> SPTPLPQLPSNVRDGENNVASTFLQAFFQLWDHDRLTLIPQFYDSETTFSVVFATDSPQDPASSSCSKFSRNLNILSPRHPSTLQRLFVGSNLIADLWKVLPATRHPSLDQTSQWLIDCHTFPHLADPTGMAPYAMGLMINVNGQCEEADISQNLYGTRTFSRCFILGPSKPGAPHPYRVLSDQLTLHTWKPQ;> MLSRRYAAKSFVEWYYRQINENKPVASGYVNNNATYTKAGHPPADITINGRVVATPEEWDTMLKEQRAQHNTSSSSTLPIGRKPVRYDVDCFDVHVINADYRFAAPQRMIEQHAPTDGVRMMMALTVSGSVYFGASPRSTDDYV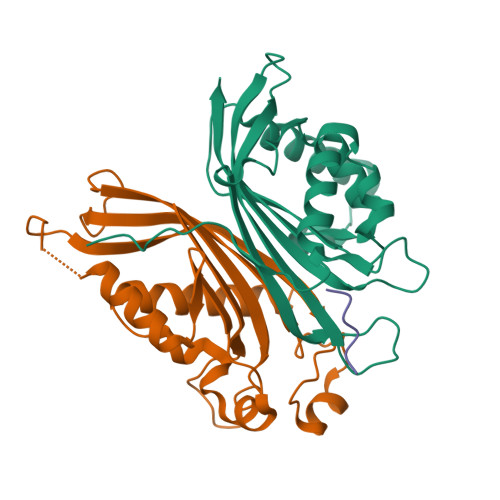IKQHFNDVFILVPNWDVLEKPGARSGRKYLIASHKYRAY;> MMAPANNPFGAPPAQVNNPF> HHHHHHENLYFQGMDIIFYHPTFDTQWWIEALRKAIPQARVRAWKSGDNDSADY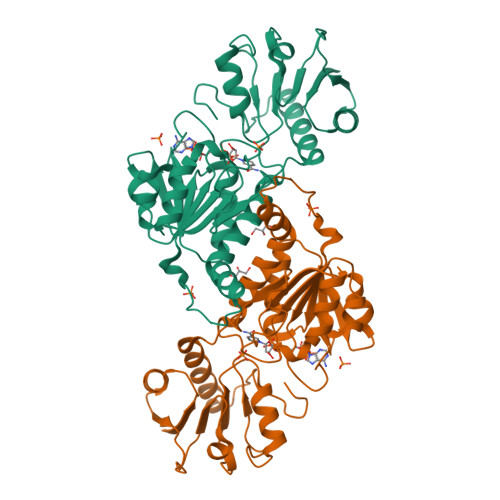ALVWHPPVEMLAGRDLKAVFALGAGVDSILSKLQAHPEMLNPSVPLFRLEDTGMGEQMQEYAVSQVLHWFRRFDDYRIQQNSSHWQPLPEYHREDFTIGILGAGVLGSKVAQSLQTWRFPLRCWSRTRKSWPGVQSFAGREELSAFLSQCRVLINLLPNTPETVGIINQQLLEKLPDGAYLLNLARGVHVVEDDLLAALDSGKVKGAMLDVFNREPLPPESPLWQHPRVTITPHVAAITRPAEAVEYISRTIAQLEKGEKVCGQVDRARGY>GPL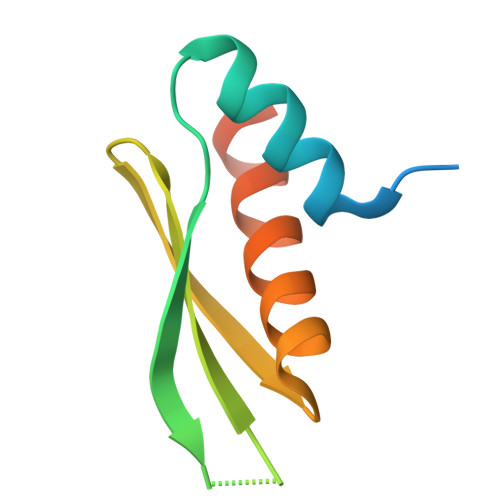GSHMLAANPGKTPISLLQEYGTRIGKTPVYDLLKAEGQAHQPNFTFRVTVGDTSCTGQGPSKKAAKHKAAEVALKHLKGGSMLEPAL[2x]> SSLEEKIEELVKELIKHTEELRRLLEKLVKEGGASEEYLLELLENLVRLARVIAEVAREQGNEELLEEAARLAEEAARQAEELAREARYEGDLELAL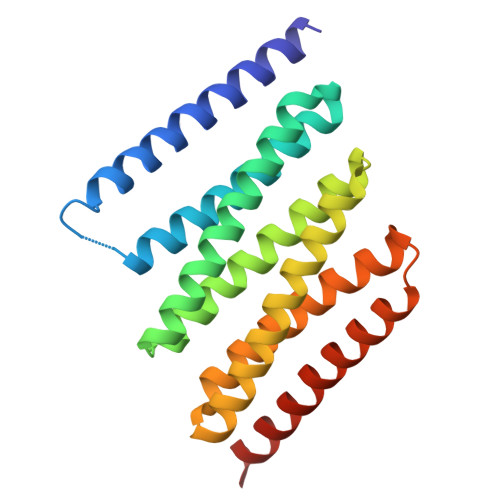KALQILVNAARVLAEIARDRGNEELLQKAAELAKEAARQAEEIAKEARERGNFELALEALEILNEAARVLARIAHHRGNQELLEEAWRLTHRSAKWSREIAEQARKEGE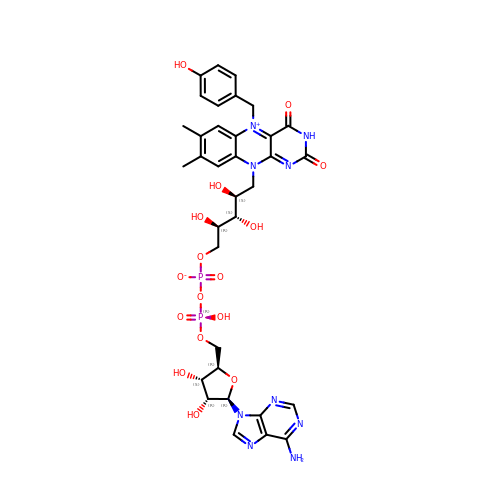N5-(4-HYDROXYBENZYL)FLAVIN-ADENINE DINUCLEOTIDE | C34 H39 N9 O16 P2 | MEBQXAOFZPAVFQ-RAWNUJITSA-N>[2x]MAMITGGELVVRTLIKAGVEHLFGLHGAHIDTIFQ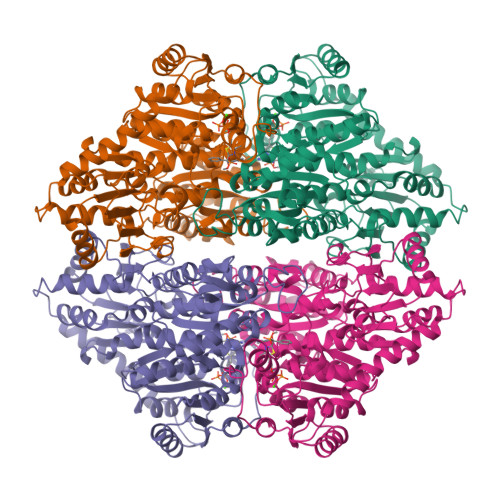ACLDHDVPIIDTRHEAAAGHAAEGYARAGAKLGVALVTAGGGFTNAVTPIANAWLDRTPVLFLTGSGALRDDETNTLQAGIDQVAMAAPITKWAHRVMATEHIPRLVMQAIRAALSAPRGPVLLDLPWDILMNQIDEDSVIIPDLVLSAHGARPDPADLDQALALLRKAERPVIVLGSEASRTARKTALSAFVAATGVPVFADYEGLSMLSGLPDAMRGGLVQNLYSFAKADAAPDLVLMLGARFGLNTGHGSGQLIPHSAQVIQVDPDACELGRLQGIALGIVADVGGTIEALAQATAQDAAWPDRGDWCAKVTDLAQERYASIAAKSSSEHALHPFHASQVIAKHVDAGVTVVADGALTYLWLSEVMSRVKPGGFLCHGYLGSMGVGFGTALGAQVADLEAGRRTILVTGDGSVGYSIGEFDTLVRKQLPLIVIIMNNQSWGATLHFQQLAVGPNRVTGTRLENGSYHGVAAAFGADGYHVDSVESFSAALAQALAHNRPACINVAVALDPIPPEELILIGMDPFGSHHHHHH> PKALIVYGSTTGNTEYTAETIARELADAGYEVDSRDAASVEAGGLFEGFDLVLLGCSTWA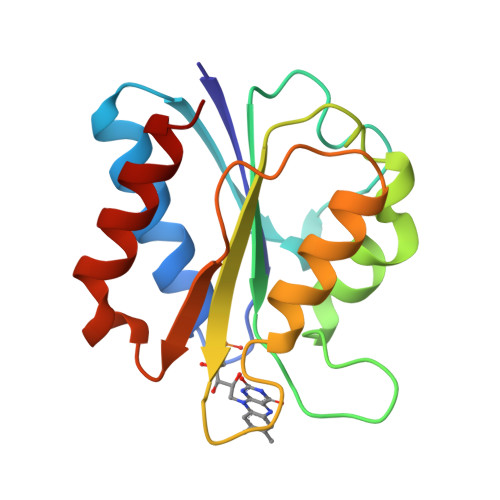DDSIELQDDFIPLFDSLEETGAQGRKVACFGCGDSSYEYFCGAVDAIEEKLKNLGAEIVQDGLRIDGDPRAARDDIVGWAHDVRGAI> GMKTIFSGIQPSGVITIGNYIGALRQFV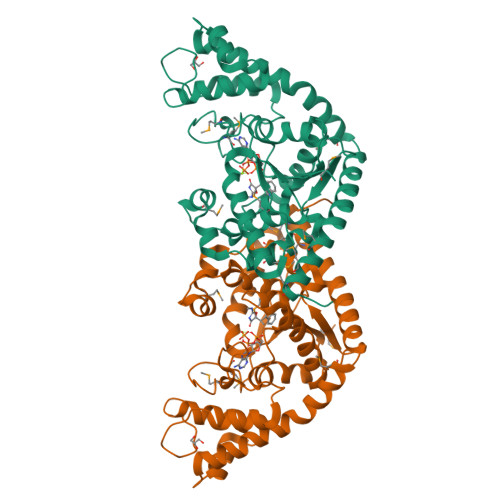ELQHEYNCYFCIVDQHAITVWQDPHELRQNIRRLAALYLAVGIDPTQATLFIQSEVPAHAQAAWMLQCIVYIGELERMTQFKEKSAGKEAVSAGLLTYPPLMAADILLYNTDIVPVGEDQKQHIELTRDLAERFNKRYGELFTIPEARIPKVGARIMSLVDPTKKMSKSDPNPKAYITLLDDAKTIEKKIKSAVTDSEGTIRYDKEAKPGISNLLNIYSTLSGQSIEELERQYEGKGYGVFKADLAQVVIETLRPIQERYHHWMESEELDRVLDEGAEKANRVASEMVRKMEQAMGLGRRR>TAAEIAALPRQKVELVDPPFVHAHSQVAEGGPKVVEFTMVIEEKKIVIDDAGTEVHAMAFNGTVPGPLMVVHQDDYLELTLINPETNTLTHNIDFHAATGALGGGGLTEINPGEKTILRFKATKPGVFVYHCAPPGMVPWHVVSGMNGAIMVLPREGLHDGKGKALTYDKIYYVGEQDFYVPRDENGKYKKYEAPGDAYEDTVKVMRTLTPTHVVFNGAVGALTGDKAMTAAVGEKVLIVHSQANRDTRPHLIGGHGDYVWATGKFNTPPDVDQETWFIPGGAAGAAFYTF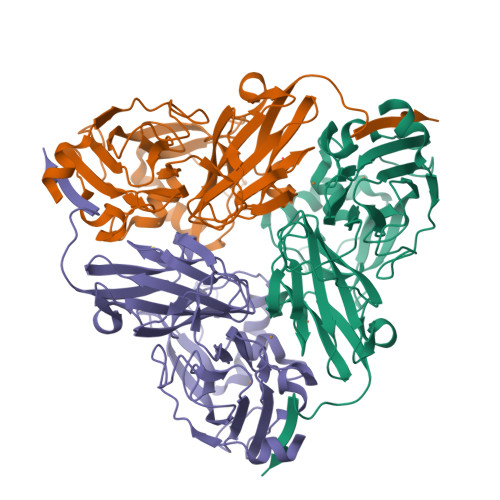QQPGIYAYVNHNLIEACELGAAAHFKVTGEWNDDLMTSVLAPSG[3x]>HHHHHHSSGLVPRGSHMAKSPELDRVIGMIRERAATPYKHL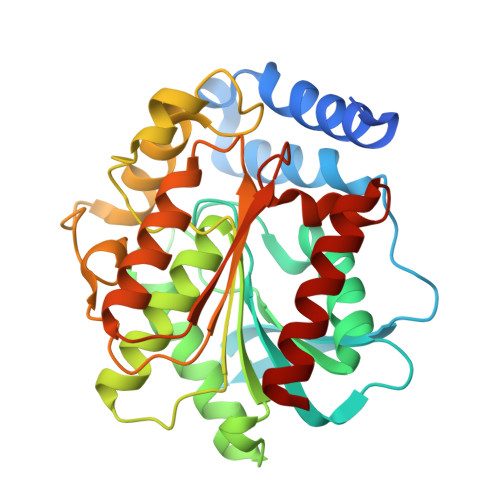STDDDRRLYETMLGSMPLDDDIQTERLGVNGVPAEWIYAPGARDDQVFLYLHGGGYVIGSMRTHRVMLSHIARAAGCRVLGLDYRLAPETPFPAPVEDTVAAYRWLLAHGYDPSRIALGGDSAGGGLVVAALVALRYIGEPLPAAGVCLSPWIDMEATGESFTTNATMDPSVNKERVMWFAALYLGGKNPQAPLASPLYADLQGLPPLLVQVGGIETLLDDARALTTRAKAAGVDADLEVWDDMPHVWQHFAPILPEGKQAIARIGEFLRKQIG[4x]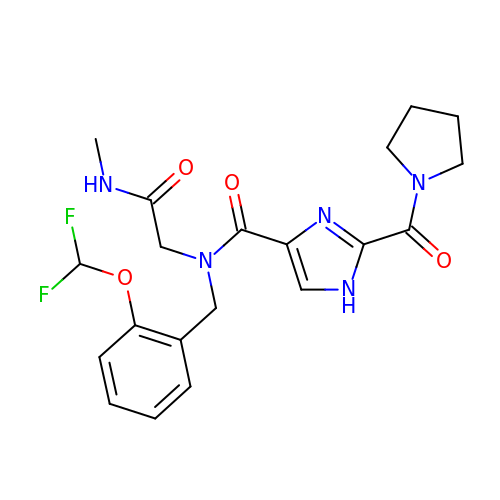~{N}-[[2-[bis(fluoranyl)methoxy]phenyl]methyl]-~{N}-[2-(methylamino)-2-oxidanylidene-ethyl]-2-pyrrolidin-1-ylcarbonyl-1~{H}-imidazole-4-carboxamide | C20 H23 F2 N5 O4 | UHBFOFSFPSKTRS-UHFFFAOYSA-N> SSAPRFLT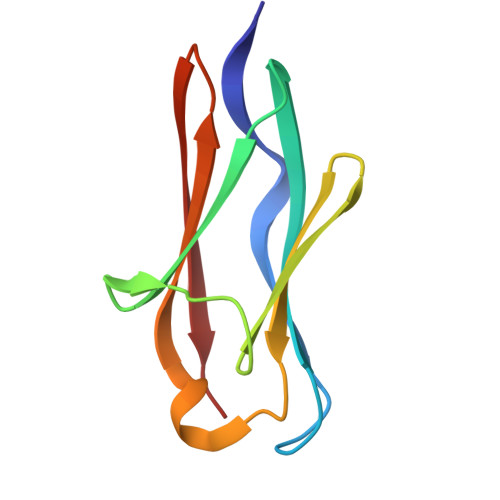RPKAFVVSVGKDATLSCQIVGNPTPQVSWEKDQQPVAAGARFRLAQDGDLYRLTILDLALGDSGQYVCRARNAIGEAFAAVGLQV> EPASTLEG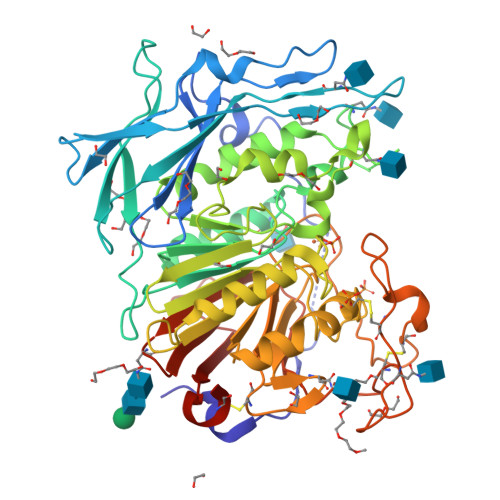PSRPVTVPLREDRGHAVDLPDTDPRVQRRVTGWAPEQIAVALSAAPTSAWVSWITGDFQMGGAVKPLDPGTVGSVVRYGLAADSLVREATGDALVYSQLYPFEGLQNYTSGIIHHVRLQGLEPGTKYYYQCGDPSIPGAMSAVHAFRTMPAVGPRSYPGRIAVVGDLGLTYNTTSTVEHMASNQPDLVLLLGDVSYANLYLTNGTGTDCYSCSFAKSTPIAETYQPRWDYWGRYMEPVTSSTPMMVVEGNHEIEQQIGNKTFAAYSARFAFPSMESESFSPFYYSFDAGGIHFIMLAAYADYSKSGEQYRWLEKDLAKVDRSVTPWLVAGWHAPWYSTYKAHYREAECMRVAMEELLYSYGLDIVFTGHVHAYERSNRVFNYTLDPCGAVHISVGDGGNREKMATTHADDPGRCPEPMSTPDAFMGGFCAFNFTSGPAAGSFCWDRQPDYSAYRESSFGHGILEVKNETHALWKWHRNQDLYQGAVGDEIYIVREPERCLLKHHHHHH> DKMDYDFKVKLSSERERVEDLFEYEGCKVGRGTYGHVYKAKRKDGKDDKDYALKQIEGTGISMSACREIALLRELKHPNVISLQKVFLSHADRKVWLLFDYAEHDLWHIIKFHRASKANKKPVQLPRGMVKSLLYQILDGIHYLHANWVLHRDLKPANILVMGEGPERGRVKIADMGFARLFNSPLKPLADLDPVVVTFWYRAPELLLGARHYTKAIDIWAIGCIFAELLTSEPIFHCRQEDIKTSNPYHHDQLDRIFNVMGFPADKDWEDIKKMPEHSTLMKDFRRNTYTNCSLIKYMEKHKVKPDSKAFHLLQKLLTMDPIKRITSEQAMQDP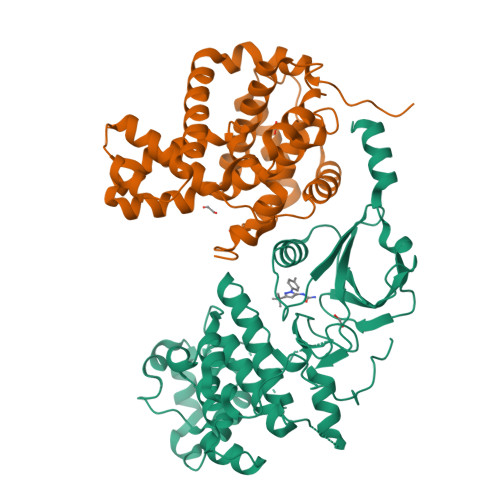YFLEDPLPTSDVFAGCQIPYPKREFLTEEEPDDKGDKKNQQQQQGNNHTNGTGHPGNQDSSHTQGPPLKK;> DDKAMAGNFWQSSHYLQWILDKQDLLKERQKDLKFLSEEEYWKLQIFFTNVIQALGEHLKLRQQVIATATVYFKRFYARYSLKSIDPVLMAPTCVFLASKVEEFGVVSNTRLIAAATSVLKTRFSYAFPKEFPYRMNHILECEFYLLELMDCCLIVYHPYRPLLQYVQDMGQEDMLLPLAWRIVNDTYRTDLCLLYPPFMIALACLHVACVVQQKDARQWFAELSVDMEKILEIIRVILKLYEQWKNFDERKEMATILSKMPKPKPPPNSEGEQGPNGSQNSSYSQS>MATEVTFFDELKIDNKVDIIGNNVRGELPNIWLQYGQFKLKASGGDGTYSWYSENTSIATVDASGKVTLNGKGSVVIKATSGDKQTVSYTIKAPSYMIKVDKQAYYADAMSIC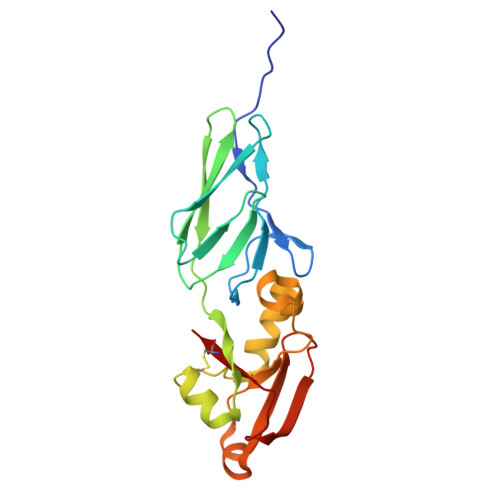KNLLPSTQTVLSDIYDSWGAANKYSHYSSMNSITAWIKQTSSEQRSGVSSTYNLITQYPLPGVNVNTPNVYAVCVE[2x]>[12x]HHHHHHGSMLFTLNDPAYLKTGLEPAISAKTLDFHFNGHHKTYLNKTNDLVKGTSLENKSLEDVILVAKTTNNAALFNNATQLWNHSFFWDCMAPTNQTGQISPELEKLIKESFGS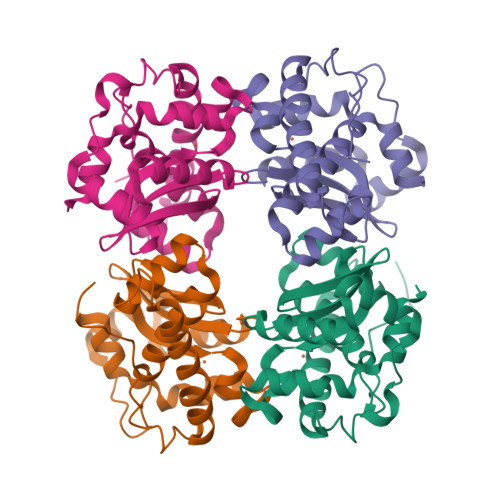VADFKKKFTDSAIANFGSGWTWLVNINGKLEIQNTSNAESPVTLRVTPLLTVDVWEHAYYLDHQNRRPEYLNKWWEVVNWKFVDQQLKQ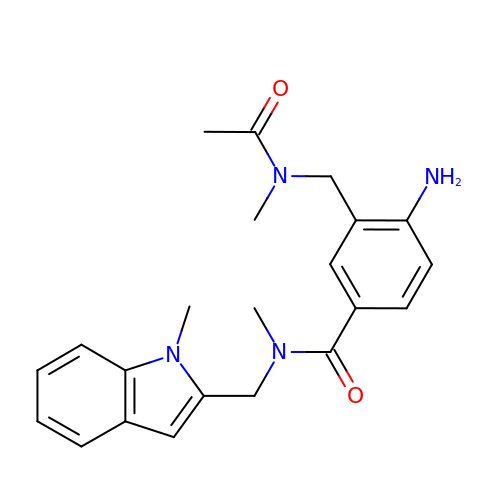3-[(ACETYL-METHYL-AMINO)-METHYL]-4-AMINO-N-METHYL-N-(1-METHYL-1H-INDOL-2-YLMETHYL)-BENZAMIDE | C22 H26 N4 O2 | AWTBJNJPBKTHEV-UHFFFAOYSA-N>MHSLMKPTREPQINLFKKSNPYKAKVISNVLLTPETGTGKRPKKEGEALVHRIVLAIDHSAYPYVIGQSGGVIPPGEDPEKKAKGLADVGYTVRLYSIASPSYSFGMKEDNIEFIIKRDNIYDENGNIQFKGVCSNYMCDLKPGDEVTMTGPSGKKFLLPNTDFSGDIMFLATGTGIAPFIGMSEELLEHKLIKFTGNITLVYGAPYSDELVMMDYLKGLESKHKNFKLITAISREEKNSFDGGRMYISHRVREQAEAVKKILNGGGRFYICGGPKGMEKGVIEEIQKISGNTGTYEEFKHHLEGAHQLFVETY[4x]

Ferredoxin-NADP(H) reductases (FNRs) are flavoenzymes that catalyze electron transfer between NADP(H) and the iron-sulfur protein ferredoxin (Fd) or flavin mononucleotide-containing flavodoxin. Leptospira interrogans FNR (LepFNR) displays low sequence identity with plant (34% with Zea mays) and bacterial (31% with Escherichia coli) FNRs. Crystal structures of LepFNR reveal a typical plastidic type reductase, analogous in its folding architecture to the enzymes found in plant and cyanobacteria, in spite of displaying an important divergence at primary structure level. Overall topology of the LepFNR molecule has the canonical FNR fold, which consists of two well defined domains, although several unique structural features were found in LepFNR 3D structure.

LepFNR·NADP+ crystal structure, refined to 2.70 Å resolution, revealed moderate structural changes when compared to LepFNR crystal structure. The high quality of electron density maps, allowed the unambiguously positioning of the NADP+ molecule noncovalently bound to the C-terminal domain of LepFNR. Small, but distinct, structural rearrangements could be identified upon NADP+ binding. Tyr247 changes its side-chain conformation and bends toward the NADP+ in LepFNR·NADP+ crystal structure, thus facilitating interactions between adenine phosphate and its side chain hydroxyl group. NADP+ binding also causes changes in Arg245 conformation, which also is part of the NADP+ binding site. NADP+ molecule is attached to LepFNR C-terminal domain by a network of hydrogen bonds. The phosphate group is anchored by the hydrogen bonds with Arg245 and Arg235. At variance, in LepFNR the nicotinamide portion of NADP+ makes water mediated hydrogen bonds with Asp119, Arg41 and Glu210. The overall structural adjustments induced by NADP+ binding in LepFNR structure are modest, and RMSD deviations between NADP+ bound and NADP+-free states are of 0.453 Å as calculated for Cα positions only. Here, the position adopted by the NADP+ nicotinamide bound to the LepFNR enzyme may represent another intermediate before the productive binding of the substrate.>[2x]QYDDSPVFTNSTYTVVVEENLPAGTSFLQIEAKDVDLGANVSYRIRSPEVKHLFALHPFTGELSLLRSLDYEAFPDQEASITFLAEAFDIYGTMPPGIATVTVIVKDMNDYPPVFSKRIYKGMVAPDAVKGTPITTVYAEDADPPGMPASRVRYRVDDVQFPYPASIFDVEEDSGRVVTRVNLNEEPTTIFKLVVVAFDDGEPVMSSSATVRILVLHPGEIPRFTQEEYRPPPVSELAARGTVVGVISAAAINQSIVYSIVAGNEEDKFGINNVTGVIYVNSPLDYETRTSYVLRVQADSLEVVLANLRVPSKSNTAKVYIEIQDENDHPPVFQKKFYIGGVSEDARMFASVLRVKATDRDTGNYSAMAYRLIIPPIKEGKEGFVVETYTGLIKTAMLFHNMRRSYFKFQ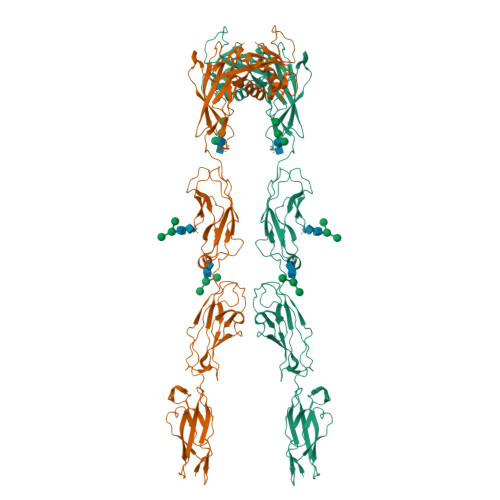VIATDDYGKGLSGKADVLVSVVNQLDMQVIVSNVPPTLVEKKIEDLTEILDRYVQEQIPGAKVVVESIGARRHGDAYSLEDYSKCDLTVYAIDPQTNRAIDRNELFKFLDGKLLDINKDFQPYYGEGGRILEIRTPEAVTSIKKRGESLGYTEGALLALAFIIILCCIPAILVVLVSYRQFKVRQAECTKTARIQSAMPAAKPAAPVPAAPAPPPPPPPPPPGAHLYEELGESAMHKYETALFESRLVPR>SGSGNNLEEEVHKLLWELSEIYHHHDHEASHEALRRALEVLKQLLEHNNLEQAVTLVSIAVHVAVRVNDEHVIRELRHFLRRLLKQVKEHNNNKLALLVMSVKMQLDRT[2x];>KAMHVAQPAVVLASSRGIASFVCEYASPGKATEVRVTVLRQADSQVTEVCAATYMMGNELTFLDDSICTGTSSGNQVNLTIQGLRAMDTGLYICKVELMYPPPYYLGIGNGTQIYVIDPEPCPDSD[2x]

We reasoned that to enable systematic design of binders to convex protein target sites it would be necessary to generate scaffold sets with overall concave shapes. We focused on 5 helix bundle scaffolds with three helices forming the concave interface and two helices providing structural support. The selected 7476 scaffolds, which we refer to as 5HCS (5 helix concave scaffolds) throughout the remainder of the text, have a wide range of curvatures. Our method for computationally designing small but concave proteins to bind to convex protein target sites expands the space of the protein surfaces that can be targeted by de novo protein design.

Immunoglobulin domain recognition plays important roles in immune receptor functions; in particular the cancer immunotherapy targets Cytotoxic--T--lymphocyte--antigen--4 (CTLA-4) have extracellular Ig fold domains that are the targets of therapeutic antibodies. The highest affinity optimized binder, 5HCS_CTLA4_1 has a sequence similarity of 82.86% compared to 5HCS_CTLA4_0. 5HCS_CTLA4_1 had an off rate too slow and a binding affinity for CTLA-4 too tight (<100 pM) to be measurable by biolayer interferometry. We determined co-crystal structures of 5HCS_CTLA4_1 with CTLA-4 and unbound crystal structures of 5HCS_CTLA4_2. The design model of 5HCS_CTLA4_1 in complex with CTLA-4 also closely agrees with the crystal structure, with a very low rmsd of 0.34 Å. 5HCS_CTLA4_1 binds to the CD86 binding site on CTLA-4 using a concave binding surface formed by H1, H3 and H5 covering both the CTLA-4 beta-turn (L98 to Y104) and hydrophobic pocket which interacts with CD86. H1 interacts with the hydrophobic beta-turn (L128 to Y136) through hydrophobic interactions between Y18 and M135 and aromatic interactions between H19 and Y136. S54 and I55 on H3 interact with Y139 on CTLA-4, and N89 on H5 hydrogen bonds with Q90 on CTLA-4. We co-cultured the cells with a range of concentrations of the CTLA–4 binder, and observed dose-dependent activation of CTLA-4 effector cells with an EC50 of 53.3 nM.methyl N-(3-hydroxy-9,10-dioxo-9,10-dihydroanthracene-2-sulfonyl)glycinate | C17 H13 N O7 S | 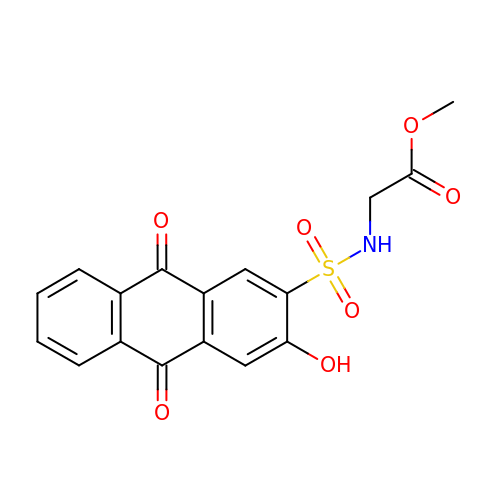ICZKTIFKJAHTGW-UHFFFAOYSA-N> AASGVATNTPTANDEEYITPVTIGGTTLNLNFDTGSADLWVFSTELPASQQSGHSVYNPSATG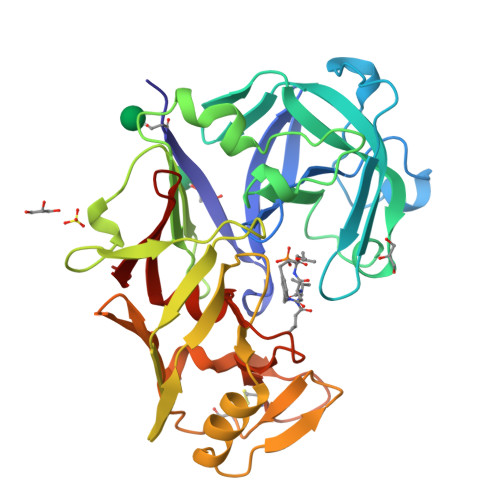KELSGYTWSISYGDGSSASGNVFTDSVTVGGVTAHGQAVQAAQQISAQFQQDTNNDGLLGLAFSSINTVQPQSQTTFFDTVKSSLAQPLFAVALKHQQPGVYDFGFIDSSKYTGSLTYTGVDNSQGFWSFNVDSYTAGSQSGDGFSGIADTGTTLLLLDDSVVSQYYSQVSGAQQDSNAGGYVFDCSTNLPDFSVSISGYTATVPGSLINYGPSGDGSTCLGGIQSNSGIGFSIFGDIFLKSQYVVFDSDGPQLGFAPQA> MESLPVIAAPSMWTRPQIRDFKEKIRQDSDSVITVGRGEVVTVRVPTHEEGSYLFWEFATDNYDIGFGVYFEWTDSPNTAVSVHVSESSEHDDEEE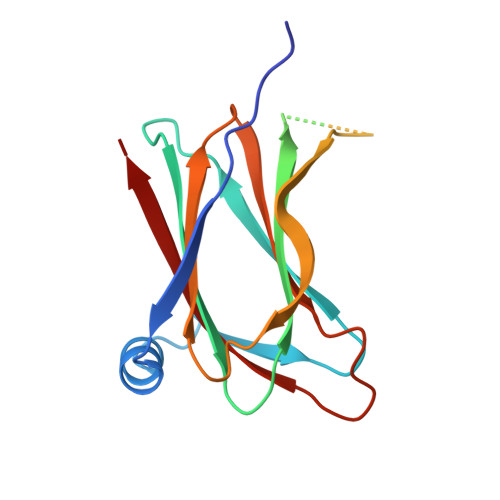EENISSEEKAKKNANKPVLDEIVPVYRRDCHEEVYAGSHQYPGRGVYLLKFDNSYSLWRSKSVYYRVYYTR> QDLMASGNTTVKATFGKDSSVVKWVVLAEVLVGAVMYMMTKNVKFLAG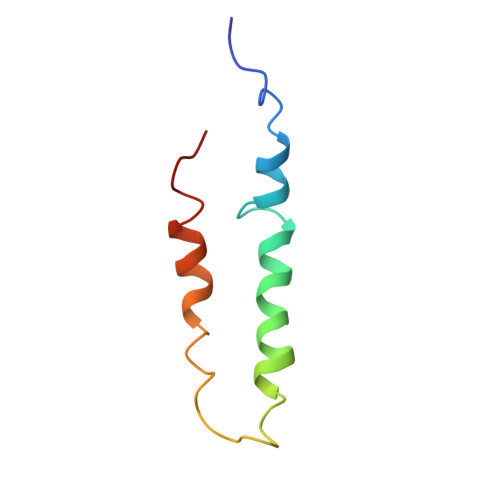FAIISVFIAVGMAVVGL> GRGK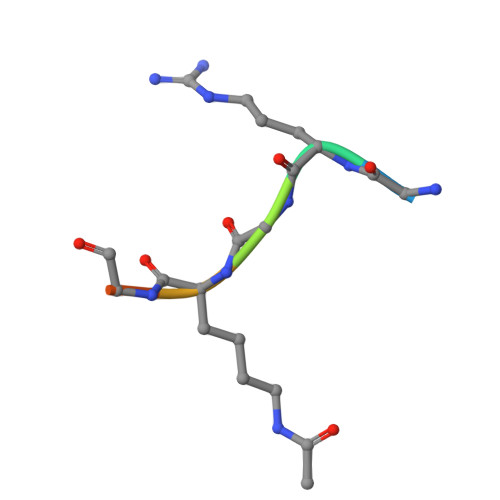GGK> RSGAPGDAALPEPNIFLIFSHGLQGCLEAQGGQVRVTPACNTSLPAQRWKWVSRNRLFNLGTMQCLGTGWPGTNTTASLGMYECDREALNLRWHCRTLGDQLSLLLGARTSNISKPGTLERGDQTRSGQWRIYGSEEDLCALPYHEVYTIQGNSHGKPCTIPFKYDNQWFHGCTSTGREDGHLWCATTQDY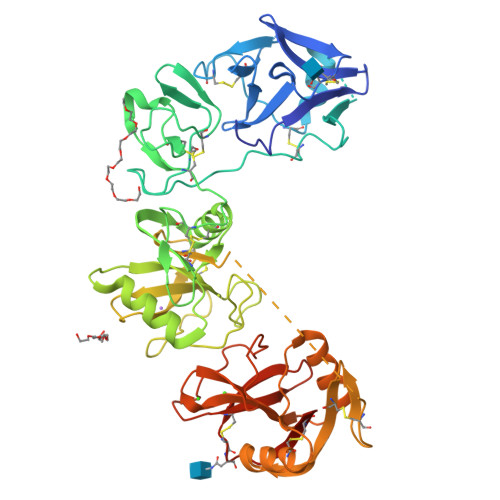GKDERWGFCPIKSNDCETFWDKDQLTDSCYQFNFQSTLSWREAWASCEQQGADLLSITEIHEQTYINGLLTGYSSTLWIGLNDLDTSGGWQWSDNSPLKYLNWESDQPDNPSEENCGVIRTESSGGWQNRDCSIALPYVCKKKPNATAEPTPPDRWANVKVECEPSWQPFQGHCYRLQAEKRSWQESKKACLRGGGDLVSIHSMAELEFITKQIKQEVEELWIGLNDLKLQMNFEWSDGSLVSFTHWHPFEPNNFRDSLEDCVTIWGPEGRWNDSPCNQSLPSICKKAGQLTRTGHHHHHH>[4x]DDLDAIQLKLQELLASLHIFYSNLRGIHWNIKDTNFFVIHKKTQKLYEYIEKIIDIVAERSRMLGYDSEFRYSEFMKKSFIKELDIESTSNFLPSMESIV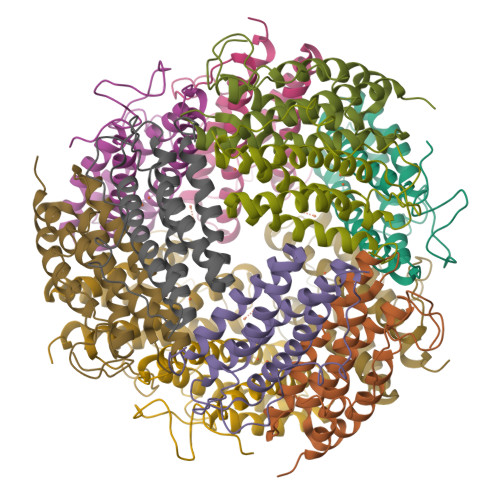CSLTEILKNIFGMRKLIDTAGDYGTANIMDDIMSDLEKHLWMHKALLENCD> MGHHHHHHMELKASEFGVVLSVDALKLSRQ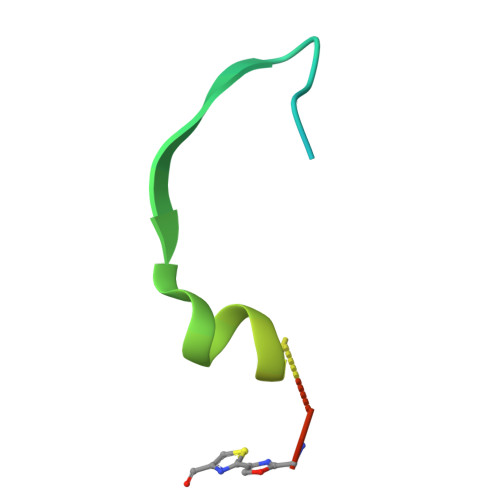SPLGVGIGGGGGGGGGGSCGGQGG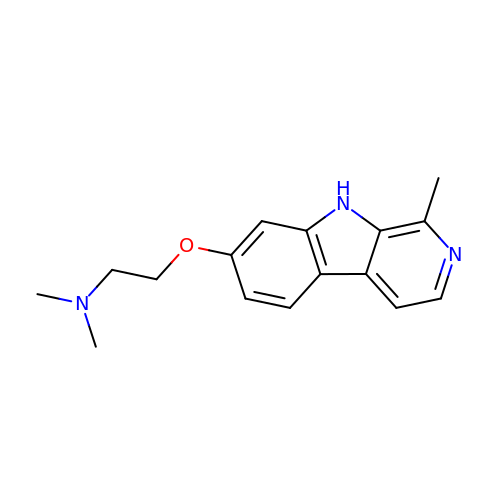~{N},~{N}-dimethyl-2-[(1-methyl-9~{H}-pyrido[3,4-b]indol-7-yl)oxy]ethanamine | C16 H19 N3 O | RMAYMVOWWDYRGB-UHFFFAOYSA-N>UUGCGUCGCUCCGGAA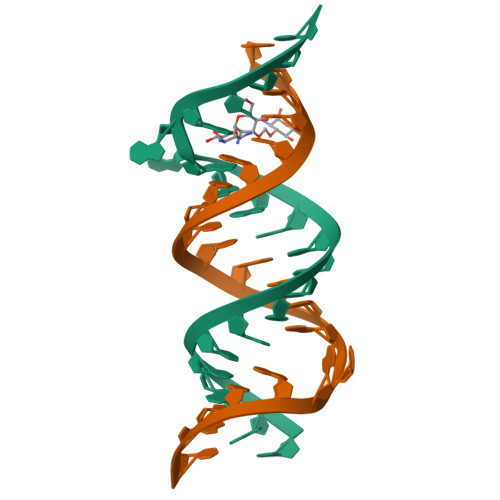AAGUCGC[2x]>[4x]ASLFPPGLHAIYGECRRLYPDQPNPLQVTAIVKYWLGGPDPLDYVSMYRNVGSPSANIPEHWHYISFGLSDLYGDNRVHEFTGTDGPSGFGFELTFRLKRETGESAPPTWPAELMQGLAR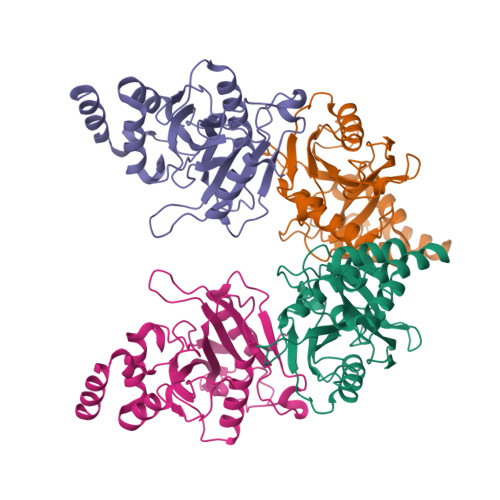YVFQSENTFCSGDHVSWHSPLDNSESRIQHMLLTEDPQMQPVQTPFGVVTFLQIVGVCTEELHSAQQWNGQGILELLRTVPIAGGPWLITDMRRGETIFEIDPHLQERVDKGIETD> GPLGSASKPEVTVRLNVHKVTVLTLQDKIVKEKFAMVAPDVQIEDGKGTILISSEEGETEANNHKKL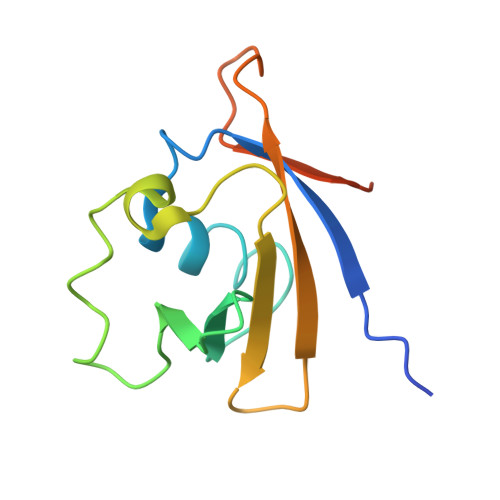SEFGIRNGSRLQADDFLQDYTLLINILHSEDLGKDVEFEVVGDAPEKVGPKQAED>NRLSVKLPGLDLKNPIIPASGCFGFGEEYAKYYDLNKLGSIMVKAT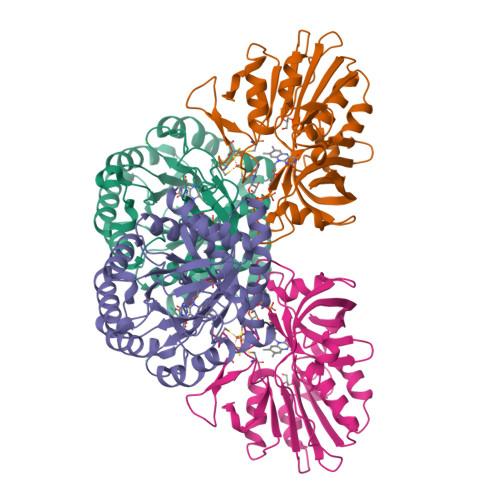TLHPRFGNPTPRVAETASGMLNAIGLQNPGLEVIMAEKLPWLNENFPDLPIIANVAGSEEDDYVAVCAKIGDAPNVKVIELNISCPNVKHGGQAFGTDPDVAAALVKACKAVSKVPLYVKLSPNVTDIVPIAKAVEAAGADGLTMINTLMGVRFDLKTRKPVLANITGGLSGPAIKPVALKLIHQVAQVVDIPIIGMGGVESAQDVLEMYMAGASAVAVGTANFADPFVCPKIIEKLPEVMDQYGIDSLENLIQEVKNSK[2x];>[2x]MPKLQEMMTIVSQREVASNIFEMVLKGELVEEMDLPGQFLHLAVPNASMLLRRPISISSWDKVAKTCTILYRIGDETSGTYEISKLQSGAKIDVMGPLGNGFPVDEVVSTDKILIVGGGIGVPPLYELAKQLEEKNCQMTILLGFASEKVKILEKEFAELKNVSLKIATDDGSYGTKGHVGMLMEEIDFEVDALYTCGAPAMLKAVAKKYEQLERLYISMESRMACGIGACYACVEHDKEDENHALKVCEDGPVFLGKQLLL>[2x]QNVSLQPPPQQLIVQNKTIDLPAVYQLNGGEEANPHAVKVLKELLSGKQSSKKGMLISIGEKGDKSVRKYSRQIPDHKEGYYLSVNEKEIVLAGNDERGTYYALQTFAQLLKDGKLPEVEIKDYPSVRYRGVVEGFYGTPWSHQARLSQLKFYGKNKMNTYIYGPKDDPYHSAPNWRLPYPDKEAAQLQELVAVANENEVDFVWAIHPGQDIKWNKEDRDLLLAKFEKMYQLGVRSFAVFFDDISGEGTNPQKQAELLNYIDEKFAQVKPDINQLVMCPTEYNKSWSNPNGNYLTTLGDKLNPSIQIMWTGDRVISDITRDGISWINERIKRPAYIWWNFPVSDYVRDHLLLGPVYGNDTTIAKEMSGFVTNPMEHAESSKIAIYSVASYAWNPAKYDTWQTWKDAIRTILPSAAEELECFAMHNSDLGPNGHGYRREESMDIQPAAERFLKAFKEGKNYDKADFETLQYTFERMKESADILLMNTENKPLIVEITPWVHQFKLTAEMGEEVLKMVEGRNESYFLRKYNHVKALQQQMFYIDQTSNQNPYQPGVKTATRVIKPLIDRTFATVVKFFNQKFNAHLDATTDYMPHKMISNVEQIKNLPLQVKANRVLISPANEVVKWAAGNSVEIELDAIYPGENIQINFGKDAPCTWGRLEISTDGKEWKTVDLKQKESRLSAGLQKAPVKFVRFTNVSDEEQQVYLRQFVLTIEKK

The enzyme responsible for removing O-GlcNAc from proteins is O-GlcNAcase (OGA),23 which is a member of glycoside hydrolase family 84 (GH84) of the CAZy classification system. Inhibitors of O-GlcNAc hydrolase (OGA), the enzyme that removes O-GlcNAc from proteins, lead to increased O-GlcNAc levels in cells and are seeing widespread adoption in the field as a research tool used in cells and in vivo. Structures of bacterial OGA homologues, in which the active site residues are completely conserved with hOGA,34,35 show a discretely sized pocket having a volume that nicely accommodates the propyl substituent of 15d. Structural data of inhibitors in complex with an hOGA homologue reveals the basis for variation in binding among these compounds.

To assess the structural basis for this stepped decrease in potency observed on going to the 2′-aminobutylthiazoline 15e, we determined the structure of Bacteroides thetaiotaomicron, a bacterial homolog (BtGH84) of hOGA, in complex with the parent 2′-aminothiazoline 11a, the tighter binding 2′-aminopropylenethiazoline 11b, and the butyl derivative 15e, which shows greatly diminished binding. In all three structures, the respective inhibitor binds in the active site in a conserved mode with an invariant hydrogen bond pattern for the aminothiazoline moiety. Propylene derivative 11b matches the size of the pocket, requiring only a minor adjustment of the C278 rotamer and showing favorable hydrophobic interactions with W337, T310, and Y282. Thus, the size of the pocket disfavors substituents longer than three carbon units in chain length, and those inhibitors having such larger groups induce unfavorable conformational changes within the active site. We also noted that the selectivity ratio for hOGA increases as the 2′-aminoalkyl chain length increases to the three-carbon propyl (15d) and propylene (11b) derivatives, but this trend reverses once the chain length increases further, as seen for the 2′-aminobutyl analogue (15e).> GAAAAMSICPHIQQVFQNEKSKDGVLKTCNAARYILNHSVPKEKFLNTMKCGTCHEINSGATFMCLQCGFCGCWNHSHFLSHSKQIGHIFGINSNNGLLFCFKCEDYIGNIDLINDAILAKYWDDVCTKTMVPSMERRDGLSGLINMGSTCFMSSILQCLIHNPYFIRHSMSQIHSNNCKVRSPDKCFSCALDKIVHELYGALNTKQASSSSTSTNRQTGFIYL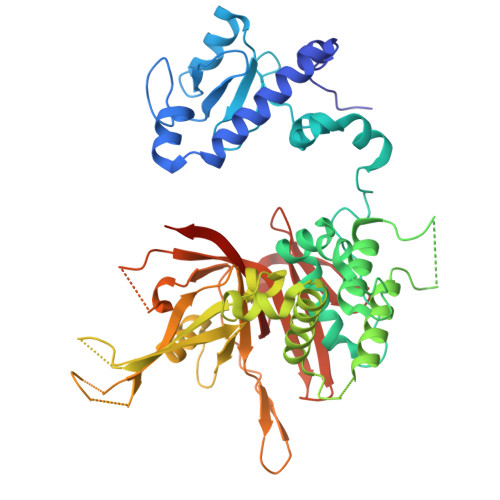LTCAWKINQNLAGYSQQDAHEFWQFIINQIHQSYVLDLPNAKEVSRANNKQCECIVHTVFEGSLESSIVCPGCQNNSKTTIDPFLDLSLDIKDKKKLYECLDSFHKKEQLKDFNYHCGECNSTQDAIKQLGIHKLPSVLVLQLKRFEHLLNGSNRKLDDFIEFPTYLNMKNYCSTKEKDKHSENGKVPDIIYELIGIVSHKGTVNEGHYIAFCKISGGQWFKFNDSMVSSISQEEVLKEQAYLLFYTIRQVN>[2x]KKWTAPFEPFQLIDNIYYVGTDGIAVYVIKTSQGLILMDTAMPQSTGMIKDNIAKLGFKVADIKLILNTHAHLDHTGGFAEIKKETGAQLVAGERDKPLLEGGYYPGDEKNEDLAFPAVKVDRAVKEGDRVTLGDTTLTAHATPGHSPGCTSWEMTVKDGKEDREVLF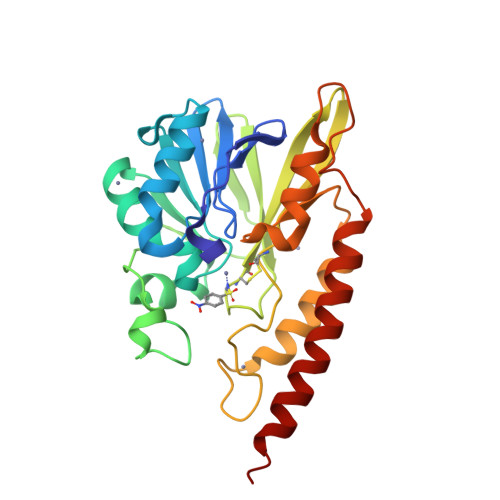FCSGTVALNRLVGQPTYAGIVDDYRATFAKAKAMKIDVLLGPHPEVYGMQAKRAEMKDGAPNPFIKPGELVTYATSLSEDFDKQLAKQTAALEKK>[2x]MSILEKITSSPSECAEHITNKDSCLSKKIQKELTSFLQKKETLGCDSESCVITHPAVKAYAQQKGLDLSKELETRFKAPGPRNNTGLLTNFNIDETLQRWAIKYTKFFNCPFSMMDFER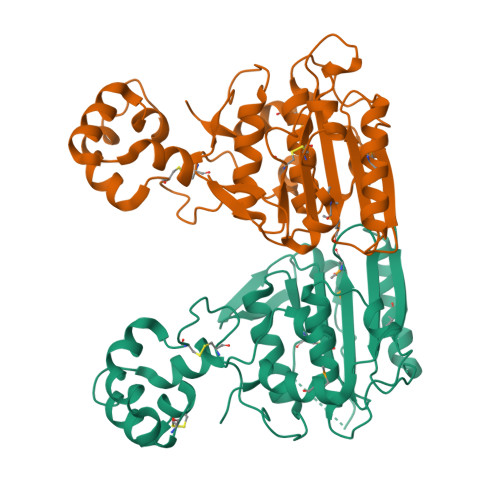IHYKFNQVDMVKVYKGEELQYVEGKAVKRPCNTFGCVLNTDFSTGTGKHWVAIFVDMRGDCWSIEYFNSAGNSPPGPVIRWMERVKQQLLKIHHTVKTLAVTNIRHQRSQTECGPYSLFYIRARLDNVSYTHFISTRITDEEMYKFRTHLFRIALEHHHHHH> MAGLPRRIIKETQRLLAEPVPGIKAEPDESNARYFHVVIAGPQDSPFEGGTFKLELFLPEEYPMAAPKVRFMTKIYHPNVDKLGRICLDILKDKWSPALQIRTVLLSIQALLSAPNPDDPLANDVAEQWKTNEAQAIETARAWTRLYAMNNI;> SHSGFKCPICSKSVASDEMEMHFIMCLSKPRLSYNDDVLTKDAGECVICLEELLQGDTIARLPCLCIYHKSCIDSWFEVNRSCPEHPA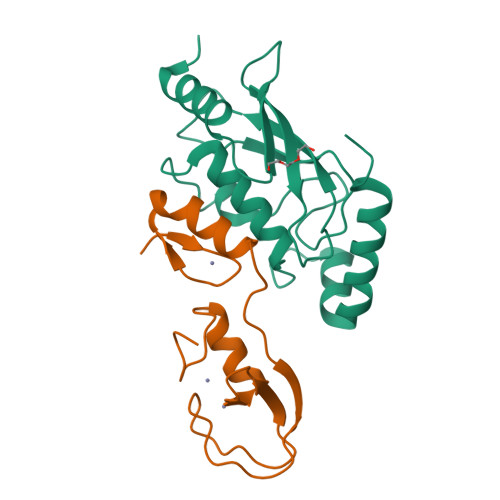D>GPGSMTTNAAHTTEQLKLGYIGLGNMGAPMATRMTEWPGGVTVYDIRIEAMTPLAEAGATLADSVADVAAADLIHITVLDDAQVREVVGELAGHAKPGTVIAIHSTISDTTAVELARDLKARDIHIVDAPVSGGAAAAARGELATMVGADREVYERIKPAFKHWAAVVIHAGEPGAGTRMKLARNMLTFTSYAAACEAMKLAEAAGLDLQALGRVVRHTDALTGGPGAIMVRDNMKDLEPDNFLYQPFLHTRGLGEKDLSLALALGEAVSVDLPLARLAYEGLAAGLGVP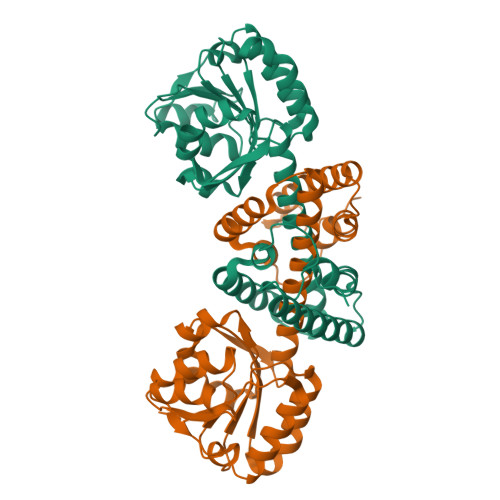HKEKEA[2x]5-(2-hydroxyethyl)nonane-1,9-diol | C11 H24 O3 | 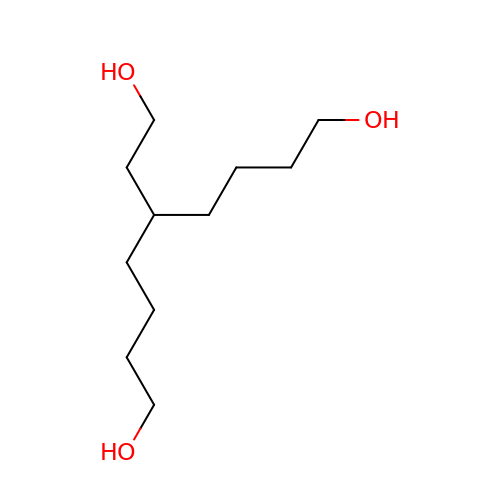VICIXNZSEUYGFV-UHFFFAOYSA-N> DVVTYNTLIDGLAKAGRL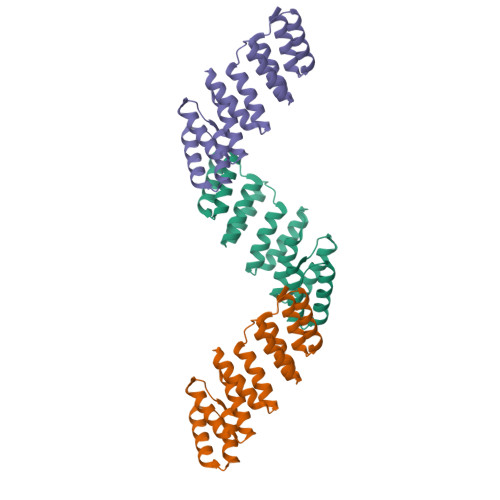EEALQLFQEMKEKGVKPDVVTYNTLIDGLAKAGRLEEALQLFQEMKEKGVKPDVVTYNTLIDGLAKAGRLEEALQLFQEMKEKGVKPDVVTYNTLIDGLAKAGRLEEALQLFQEMKEKGVKPDVVTYNTLIDGLAKAGRLEEALQLFQEMKEKGVKP> MSASAELEPDVKGRILDAAADAFMARGFANTTIDDIADEVGATKGLIYYHFRSKFDIFLAVYEDGMRRVRERVEPHSTAPGTGHQRLEAMSIAHLENLMTELGYHHVVHQGVRHQDSTALKVRQRDALTALNELRRDYERMFRRVIAEGIADGSLRRVDEALATRTLLSNLNAVDVWYRKIEGQTGEEIRELASQVVDMLIGGLAD

The mycobacterial repressor, DarR, a TetR family regulator (TFR), was the first transcription regulator shown to bind c-di-AMP. Recently, DarR, a 201 residue, TFR regulator of a putative MDR transporter, Ms5347, in Mycobacteria was discovered and represents the focus of this work. Structures of TFR proteins reveal that they share a two-domain architecture with an N-terminal DNA-binding domain and a C-terminal inducer binding/dimerization domain. The DarR N-terminal domain consists of helices 1-3 and the dimer domain is comprised of helices α4-α9. In DarR, dimerization is mediated by helices α8 and α9, which interact with α8´ and α9´ (where the prime indicates the other subunit in the dimer) to form a four-helix bundle dimerization module.

The M. baixiangningiae DarR structure was solved by selenomethionine single wavelength anomalous diffraction (SAD) and refined to final Rwork/Rfree values of 18.5%/20.2% to 1.6 Å. By contrast, electron density with an unusual spirocyclic-like structure was found in the ligand-binding pocket of the M. baixiangningiae DarR structure near residues 108-138. The borate complex ligand possesses a partial negative charge, which is stabilized by an interaction with DarR residue Arg135. In addition to Arg135, there are numerous DarR residues that contact the ligand, including Met66, His94, Asn97, His105, Val108, His109, Tyr138, Leu168 and Asn172. By contrast, the HTH distance observed in the M. baixiangningiae DarR is significantly larger, 50 Å, indicative of an induced state. Consistent with this, the M. baixiangningiae DarR structure was shown to contain a bound ligand inducer. First, the shift of residues in the loop towards the dimer interface leads to a pendulum-like movement of the DNA binding domain as a unit, which leads to the large increase in the distance between DNA binding domains. Second, the structural changes in residues 117-122 prevent the formation of the cross contacts between the central subunits of the dimers in the DNA bound state, which we demonstrated is essential for the dimer-of-dimer binding mechanism.> 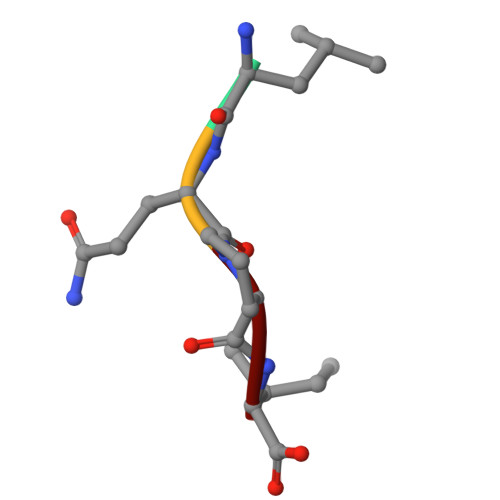LQPI>MGQIITFFQEVPHVIEEVMNIVLIALSLLAILKGIYNVATCGLFGLVSFLLLCGRSCSTTYKGVYELQTLELNMASLNMTMPLSCTKNNSHHYIMVGNETGLELTLTNTSIINHKFCNLSDAHKRNLYDHALMSIISTFHLSIPNFNQYEAMSCDFNGGKISVQYNLSHTYAVDAAKHCGTIANGVLQTFMRMAWGGSYIALDSGCGSWDCIMTSYQYLIIQNTTWEDHCQFSRPSPIGYLGLLSQRTRDIYIS[3x];>GTFTWTLSDSEGNETPGGYCLTRWMLIEAELKCFGNTAVAKCNEKHDEEFCDMLRLFDFNKQAIRRLKAPAQMSIQLINKAVNALINDQLIMKNHLRDIMCIPYCNYSKYWYLNHTVTGKTSLPRCWLVSNGSYLNETHFSDDIEQQADNMITELLQKEYIDRQG[3x]

The LASV glycoprotein complex (GPC) mediates viral entry and is the sole target for neutralizing antibodies. In its mature, native form, GPC is a trimer of heterotrimers comprised of the receptor-engaging subunit GP1; the transmembrane-spanning subunit GP2, which contains the GPC’s fusion peptide at its N terminus; and the stable signal peptide (SSP), which remains non-covalently complexed near the membrane-proximal region of GP2 post-cleavage. The GPC is expressed as a single polypeptide precursor before being proteolytically processed by signal peptidase (SPase)21 followed by site-1 protease (S1P). We present the development and characterization of prefusion-stabilized, trimeric GPCs of LASV lineages II, V, and VII, revealing structural conservation despite sequence diversity.

We focus on LASV lineages of public health concern including lineage II, one of the most common lineages that circulates widely in southern Nigeria; lineage V, which circulates in Mali and has decreased pathogenicity compared with lineage IV; and lineage VII, a newly described lineage isolated from a nosocomial infection in Togo with comparable pathogenicity to lineage IV. The resulting soluble constructs feature sequences of circulating lineages II (LII; strain NIG08-A41), V (LV; strain Soromba-R), and VII (LVII; strain Togo/2016/7082). Combined, these approaches enabled us to determine the structures of GPC in a reproducible manner and yielded structures of LIV, LII, LV, and LVII GPC trimers at resolutions of 3.8, 3.7, 3.7, and 3.1 Å, respectively. LII, LV, and LVII each have an additional PNGS at residue N271 or N272, though this site is uniformly unoccupied. Similarly, when comparing the GPCs of diverse lineages, we observe high structural homology. Using the prototypical LIV GPC as reference, we note RMSDs for pruned and all sequence-aligned pair as follows: 0.78 and 1.9 (LII), 0.85 and 2.0 (LV), and 0.73 and 2.4 Å (LVII). The main differences among the GPC lineages are found in flexible loops, most notably the loop (residues 166–181) extending from the β7 sheet prior to the α3 helix. This observed heterogeneity is derived from areas in the EM map of poorer local resolution, insinuating greater flexibility of the residues in these regions. Consequently, these differences may not represent physiologically important conformational epitopes for LII, LV, and LVII GPCs. We observed neutralization of viruses pseudotyped with GPCs from LII, LIII, and LIV by both 12.1F and 19.7E, consistent with the binding data.> ACTTCCAGTCCGTGGTAGGGCAGGTTGGGGTGACCGCTATAT;> ATATAGCGTGGAAGT

pmcDNA origami is a rapidly evolving field in nanotechnology that has shown great promise for creating nanostructures created by folding a long single-stranded DNA “scaffold” into a desired shape using hundreds of short, synthetic DNA strands called staples. In this study, we examined the impact of internal crossover distribution and the compositional uniformity of staple strands on the structure of multilayer DNA origami using cryogenic electron microscopy (cryo-EM) single-particle analysis. A refined DNA object was utilized as an alignment framework in a host–guest model, where we successfully resolved an 8 kDa thrombin binding aptamer (TBA) linked to the host object. We next tested the utility of DNA origami host supports to help resolve small guest targets.

We chose a 27-base-long thrombin-binding DNA aptamer with a molecular weight of approximately 8 kDa. To incorporate the DNA aptamer, we used the DNA origami V4. At selected sites, the scaffold strand was left single-stranded for hybridization with specific handle sequences flanking the DNA aptamer (eight bases at the 3′ end and eight at the 5′ end of the aptamer sequence), and the staples were purified using HPLC. The sample was a multilayer DNA origami object termed V4 in square lattice packing produced using a custom scaffold strand with a length of 1033 bases. We used SPA to obtain a DNA origami aptamer complex structure. Figure 3B shows a representative micrograph, 2D classifications, and a consensus map of DNA origami particles at an overall resolution of 7.5 Å. The consensus identified the aptamer as a globular protrusion at the expected site. Multibody refinement was used to improve the resolution of the central domain (4.9 Å), leading to a better-resolved EM density for the DNA aptamer. As detailed in the methods, a model based on the aptamer crystal structure and double-stranded scaffold DNA could be fitted by restrained molecular dynamics (MDFF). The observed conformational change relative to the reference crystal structure could be due to the absence of the α-thrombin which was cocrystallized in a bound state with the aptamer bound but was absent in our experiments. The required resolution could not be reached in the current study, which we attribute to the residual intrinsic heterogeneity of the DNA origami host structure, as caused by interhelical breathing motions and defects, and to the flexibility of the connections between the guest molecule and DNA origami support.>MVKETHRFETFTEEPIRLIGEEGEWLGDFPLDLEGEKLRRLYRDMLAARMLDERYTILIRTGKTSFIAPAAGHEAAQVAIAHAIRPGFDWVFPYYRDHGLALALGIPLKELLGQMLATKADPNKGRQMPEHPGSKALNFFTVASPIASHVPPAAGAAISMKLLRTGQVAVCTFGDGATSEGDWYAGINFAAVQGAPAVFIAENNFYAISVDYRHQTHSPTIADKAHAFGIPGYLVDGMDVLASYYVVKEAVERARRGEGPSLVELRVYRYGPHSSADDDSRYRPKEEVAFWRKKDPIPRFRRFLEARGLWNEEWEEDVREEIRAELERGLKEAEEAGPVPPEWMFEDVFAEKPWHLLRQEALLKEEL[2x];>[2x]MALMTMVQALNRALDEEMAKDPRVVVLGEDVGKRGGVFLVTEGLLQKYGPDRVMDTPLSEAAIVGAALGMAAHGLRPVAEIQFADYIFPGFDQLVSQVAKLRYRSGGQFTAPLVVRMPSGGGVRGGHHHSQSPEAHFVHTAGLKVVAVSTPYDAKGLLKAAIRDEDPVVFLEPKRLYRSVKEEVPEEDYTLPIGKAALRREGKDLTLICYGTVMPEVLQAAAELAKAGVSAEVLDLRTLMPWDYEAVMNSVAKTGRV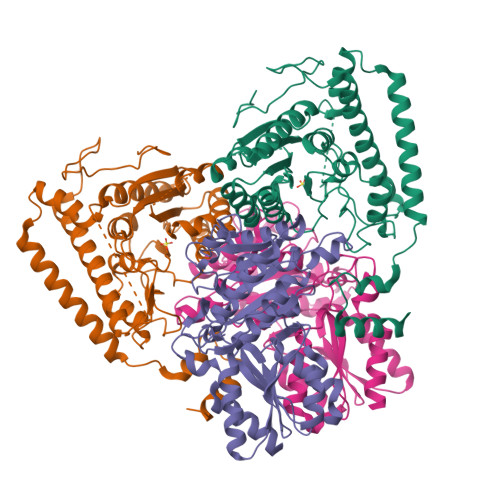VLVSDAPRHASFVSEVAATIAEDLLDMLLAPPIRVTGFDTPYPYAQDKLYLPTVTRILNAAKRALDY> LCLSQQFKAQGDYILGGLFPLGSTEEATLNQRTQPNSIPCNRFSPLGLFLAMAMKMAVEEINNGSALLPGLRLGYDLFDTCSEPVVTMKSSLMFLAKVGSQSIAAYCNYTQYQPRVLAVIGPHSSELALITGKFFSFFLMPQVSYSASMDRLSDRETFPSFFRTVPSDRVQLQAVVTLLQN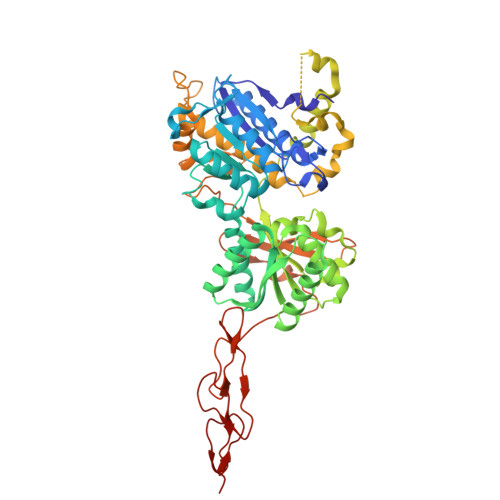FSWNWVAALGSDDDYGREGLSIFSSLANARGICIAHEGLVPQHDTSGQQLGKVLDVLRQVNQSKVQVVVLFASARAVYSLFSYSIHHGLSPKVWVASESWLTSDLVMTLPNIARVGTVLGFLQRGALLPEFSHYVETHLALAADPAFCASLNAELDLEEHVMGQRCPRCDDIMLQNLSSGLLQNLSAGQLHHQIFATYAAVYSVAQALHNTLQCNVSHCHVSEHVLPWQLLENMYNMSFHARDLTLQFDAEGNVDMEYDLKMWVWQSPTPVLHTVGTFNGTLQLQQSKMYWPGNQVPVSQCSRQCKDGQVRRVKGFHSCCYDCVDCKAGSYRKHPDDFTCTPCNQDQWSPEKSTACLPRR At the cytoplasmic face of the NPC, Nxf1•Nxt1-bound mRNPs encounter the cytoplasmic filament nucleoporins Gle1, Nup42, and Nup214, which specifically activate the DEAD-box helicase DDX19 to remove Nxf1•Nxt1 from the mRNP8. DDX19 is a member of the DEAD-box helicase family, which are RNA-dependent ATPases composed of two RecA domains (referred to as DDX19NTD and DDX19CTD throughout the text). Gle1CTD plays an important organizational role by providing spatially separated binding sites for Nup42GBM and the DEAD-box helicase DDX19/scDbp5. A comprehensive structure-function analysis of DDX19 indicates that binding of Gle1CTD•Nup42GBM induces a conformational change in DDX19, thereby stimulating its ATPase activity.

To evaluate whether the mode of interaction observed for S. cerevisiae Gle1CTD•Nup42GBM was conserved in other eukaryotes, we determined the crystal structures of human Gle1CTD•Nup42GBM at 2.8 Å resolution and of C. thermophilum Gle1CTD•Nup42GBM in the presence and absence of IP6 at 2.17 and 2.65 Å resolution, respectively. The overall structure of Gle1CTD is conserved between fungi and humans, with minor differences resulting from small insertions or different loop sizes. Both human and C. thermophilum Nup42GBM adopt the same fold as S. cerevisiae Nup42GBM and recognize the same surface on Gle1CTD, with the critical hydrophobic residues nearly universally conserved. Similarly, C. thermophilum Gle1CTD•Nup42GBM undergoes minimal conformational changes upon IP6 binding, which are mostly limited to a loop directly adjacent to the IP6 pocket. IP6 binds to C. thermophilum Gle1CTD and to S. cerevisiae Gle1CTD in a similar orientation, suggesting that IP6 could function similarly in C. thermophilum as in S. cerevisiae. The interaction between C. thermophilum Gle1CTD•Nup42GBM and Dbp5 also required IP6, consistent with the evolutionary conservation of the IP6 binding residues among fungi.

>GPHMRYVEIHRNLKGLRKYMAEQAKTNLKLKQRMGDMRREIRKSVGQLTTGGMAANKDKQQKIKSILTEALSNQVESALVDPNNFVVEPRKPVEGATNNDPLLPSIFVYLINIFAKAAISQFINEAGARPETADPVGICVAAILSEPDFLWRGASLIDILIAKFRIVCPVLFGYRGSEKTEQGRQRLGWWKESGQWISEQQHMDRMTGLGAGFAAISLRKFALSKKQNPYPPRFYWMAMAKIVNTPPAEISNTQCVVLKAMVQNYEAKFIEFYGSAAIAALRTALIDFPARAPHKSAAVNSLEVLAQMLKRDTGLDLG[2x];>GPHMGSPEFDGTLVRIWMPDGAPAYTADTEAEDPKVYEDEGVKRQWQSFLEKGRFEGGMPEVPPRREWCVWDF[2x]>MTPPPADDTSGKSGRRTELLDIAATLFAERGLRATTVRDIADAAGILSGSLYHHFDSKESMVDEILRGFLDDLFGKYREIVASGLDSRATLEALVTTSYEAIDASHSAVAIYQDEVKHLVANERFTYLSELNTEFRELWMGVLEAGVKDGSFRSDIDVELAFRFLRDTAWVAVRWYRPGGSVTVDTVAKQYLSIV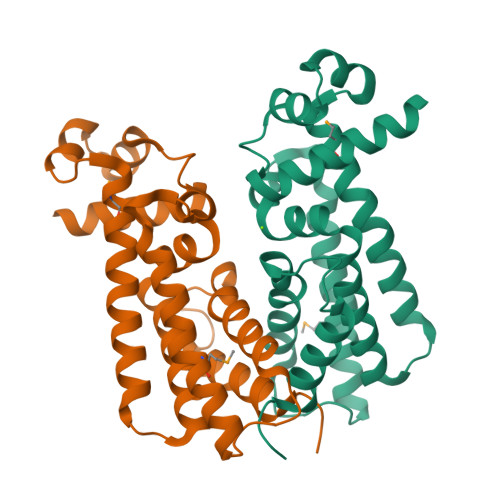LDGLASPHN[2x]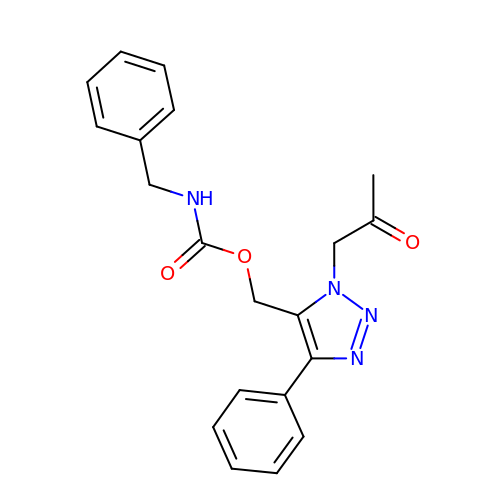[1-(2-oxopropyl)-4-phenyl-1H-1,2,3-triazol-5-yl]methyl benzylcarbamate | C20 H20 N4 O3 | WXRQXWFHRZFFIN-UHFFFAOYSA-N>MAHHHHHHMTATAQIPGGAMVQQTAGFVLSQLARHRSSWNKETMCPPLVVGVQGPQGAGKSHLTGLLPDYLEKHYGLRLATMSLDDFYLTHSDQVKLSQSEPDNPLLNGRGPAGTHDLPLLEQCLAKLKSINDRSAKFPTATKDQRAQLPIYDKSLFKGEGDRSKEVVEVQGPIDVVIFEGWMNGFGPLSNDKLEEKYAEAGRQWPSSSLVGAPGVMPTILLYSRSTLHSINQNLRQYEVLWDQIDCFVQIQPLDL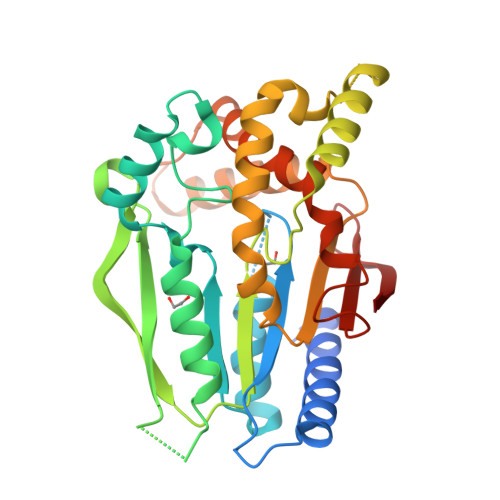SYVWTWRLQQEHNMKAKNGGNGMTDEQVRHFINRYMPSYELFQDGIDKETTSWRGKGLRFIVNIKREIVGTESF[2x]>AGVLPAHGTQHGIRLPLRSGLGGAPLGLRLPRETDEEPEEPGRRGSFVEMVDNLRGKSGQGYYVEMTVGSPPQTLNILVDTGSSNFAVGAAPHPFLHRYYQRQLSSTYRDLRKGVYVPYTQGKWEGELGTDLVSIPHGPNVTVRANIAAITESDKFFINGSNWEGILGLAYAEIARPDDSLEPFFDSLVKQTHVPNLFSLQLCGAGFPLNQSEVLASVGGSMIIGGIDHSLYTGSLWYTPIRREWYYEVIIVRVEINGQDLKMDCKEYN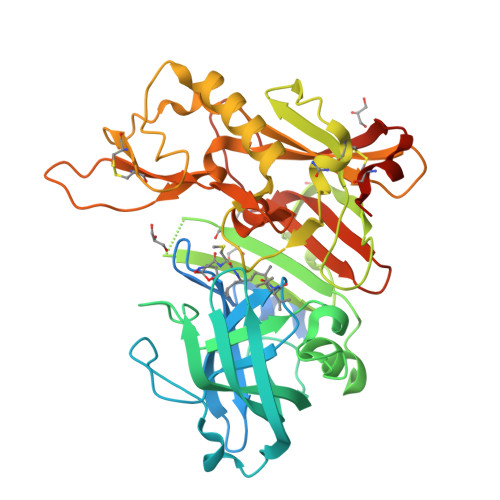YDKSIVDSGTTNLRLPKKVFEAAVKSIKAASSTEKFPDGFWLGEQLVCWQAGTTPWNIFPVISLYLMGEVTNQSFRITILPQQYLRPVEDVATSQDDCYKFAISQSSTGTVMGAVIMEGFYVVFDRARKRIGFAVSACHVHDEFRTAAVEGPFVTLDMEDCGYNIPQTDEST[3x]>KQEQPEINLDHVVEQTIKKVQQNQNQNKDPDELRSKVPGEVTASDWEALVGDTRYGYFDETGDWSWKGYFDEQGKWVWNEPVDSLEHHHHHH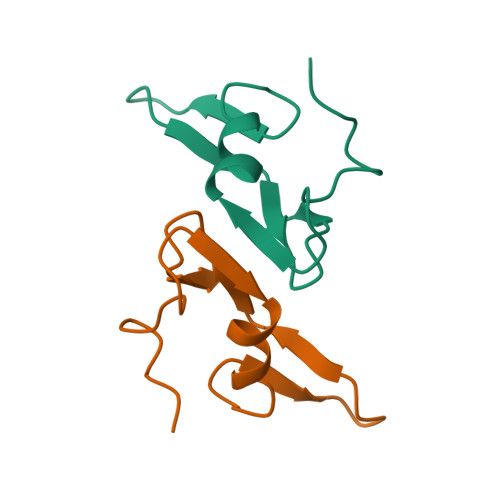[2x]> MDRDTKLAFRLRGSHSRRTDDIDDDVIVFKTPNAVYREENSPIQSPVQPILSSPKLANSFEFPITTNNVNAQDRHEHGYQPLDAEDYPMIDSENKSLISESPQNVRNDEDLTTRYNFDDIPIRQLSSSITSVTTIDVLSSLFINLFENDLIPQALKDFNKSDDDQFRKLLYKLDL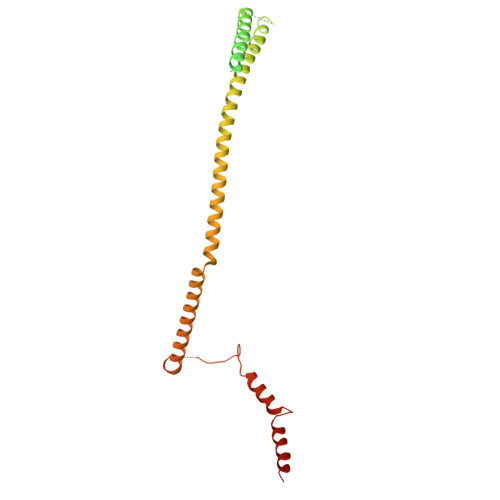RLFQTISDQMTRDLKDILDINVSNNELCYQLKQVLARKEDLNQQIISVRNEIQELKAGKDWHDLQNEQAKLNDKVKLNKRLNDLTSTLLGKYEGDRKIMSQDSEDDSIRDDSNILDIAHFVDLMDPYNGLLKKINKINENLSNEL>[2x]AYQLLLSKETLNKILQYKQNLEKGLATPGKFFLEELSKQEKSISEMDITTFTQLLIQSKKPQVFAESQVYHDGTDWTLEEESILGDVSVNMPVTMYNDGGHGSSFKNHPKPISGYLAYVPGALLASGSGPTSDMKEVLDNGKLNQDKLNALYERRLLPQLIHFNELARQNEKQAAITIPGIGTGCFSGAYYDVIKPYVRNALIHILEKHKDSLPYIDIIHYDPYMGDEPAEKKIGHMSFRVSPSGVVRGTTGQLDYPLGSNPDTHILVSIVAWDHFSWPGNDYWGGARQTDDGVKAASTDTMGQVTGATGVYDKKWGRYMPPESFTKDRKGMSDWGDYVRENGIVFNGPVLALDKSGKLDTLE

The intracellular bacterial pathogen Legionella pneumophila modulates host cell functions by secreting multiple effectors with diverse biochemical activities. In particular, effectors of the SidE family interfere with host protein ubiquitination in a process that involves production of phosphoribosyl ubiquitin (PR-Ub). Here, we show that effector LnaB converts PR-Ub into ADP-ribosylated ubiquitin, which is further processed to ADP-ribose and functional ubiquitin by the (ADP-ribosyl)hydrolase MavL, thus maintaining ubiquitin homeostasis in infected cells. The activity of LnaB requires a motif consisting of Ser, His and Glu (SHxxxE) present in a large family of toxins from diverse bacterial pathogens.

To understand the catalytic mechanism of the ADP-ribosylhydrolase (ARH) activity of MavL, we screened its active truncation mutants and succeeded in solving the structure of the MavL40-404-ADPR complex at a resolution of 2.38 Å, which revealed that several pairs of hydrogen bonds and a π-π stacking interaction provided by surrounding amino acids or water molecules are involved in interactions between MavL and ADPR. The negatively charged residues D315, D323, and D333 likely form a catalytic loop (β8-α8) that directly interacts with the hydroxyl groups of ribose by hydrogen bonding. Mutational analysis indicated that all three residues are critical for the ARH activity of MavL against ADPR-Ub. Indeed, recombinant MavL effectively hydrolyzed ADPR-Ub into ADPR and ubiquitin, which is in contrast to DupA and DupB. In addition, we observed four water molecules around the ADPR moiety, two of which (H2O-1 and H2O-2) are also found in other macro domain ARHs. These two water molecules form a hydrogen bond network with the α-phosphate of ADPR and the O1” site of the distal ribose group, wherein the α-phosphate activates H2O-1 to initiate a nucleophilic attack on the O1” glycosidic bond, leading to its cleavage (middle).>[2x]MNANDNVVIVGTGLAGVEVAFGLRAS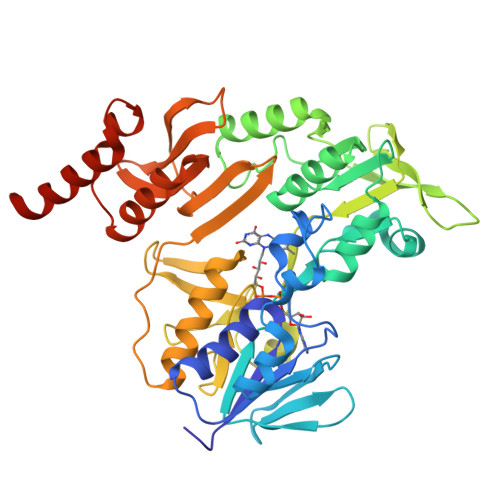GWEGNIRLVGDATVIPHHLPPLSKAYLAGKATAESLYLRTPDAYAAQNIQLLGGTQVTAINRDRQQVILSDGRALDYDRLVLATGGRPRPLPVASGAVGKANNFRYLRTLEDAECIRRQLIADNRLVVIGGGYIGLEVAATAIKANMHVTLLDTAARVLERVTAPPVSAFYEHLHREAGVDIRTGTQVCGFEMSTDQQKVTAVLCEDGTRLPADLVIAGIGLIPNCELASAAGLQVDNGIVINEHMQTSDPLIMAVGDCARFHSQLYDRWVRIESVPNALEQARKIAAILCGKVPRDEAAPWFWSDQYEIGLKMVGLSEGYDRIIVRGSLAQPDFSVFYLQGDRVLAVDTVNRPVEFNQSKQIITDRLPVEPNLLGDESVPLKEIIAAAKAELSSAPARHHHHHH>[4x]GSKGVSDLLGFKIFGMPLPLYAFALITLLLSHFYNALPTDIVGGFAIMFIIGAIFGEIGKRLPIFNKYIGGAPVMIFLV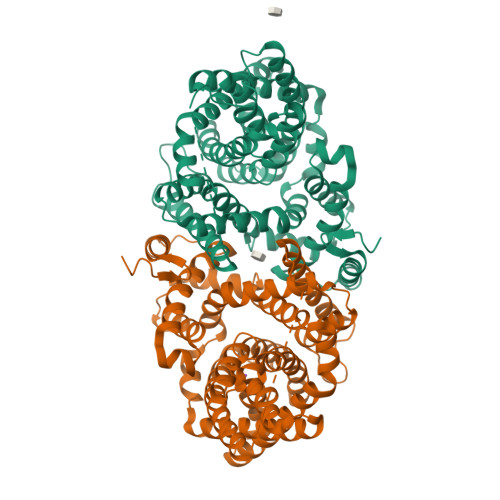AAYFVYAGIFTQKEIDAISNVMDKSNFLNLFIAVLITGAILSVNRRLLLKSLLGYIPTILMGIVGASIFGIAIGLVFGIPVDRIMMLYVLPIMGGGNGAGAVPLSEIYHSVTGRSREEYYSTAIAILTIANIFAIVFAAVLDIIGKKHTWLSGEGELVRKASFKVEEDEKTGQITHRETAVGLVLSTTCFLLAYVVAKKILPSIGGVAIHYFAWMVLIVAALNASGLCSPEIKAGAKRLSDFFSKQLLWVLMVGVGVCYTDLQEIINAITFANVVIAAIIVIGAVLGAAIGGWLMGFFPIESAITAGLCMANRGGSGDLEVLSACNRMNLISYAQISSRLGGGIVLVIASIVFGMMIPR> MHHHHHHHAVRASEISRVYEAYPEKKATLYFLVLGFLALIVGSLFGPFQALNYGNVDAYPLLKRLLPFVQSYYQGLTLHGVLNAIVFTQLFAQAIMVYLPARELNMRPNMGLMWLSWWMAFIGLVVFALPLLANEATVLYTFYPPLKGHWAFYLGASVFVLSTWVSIYIVLDLWRRWKAANPGKVTPLVTYMAVVFWLMWFLASLGLVLEAVLFLLPWSFGLVEGVDPLVARTLFWWTGHPINYFWLLPAYAIIYTILPKQAGGKLVSDPMARLAFLLFLLLSTPVGFHHQFADPGIDPTWKMIHSVLTLFVAVPSLMTAFTVAASLEFAGRLRGGRGLFGWIRAL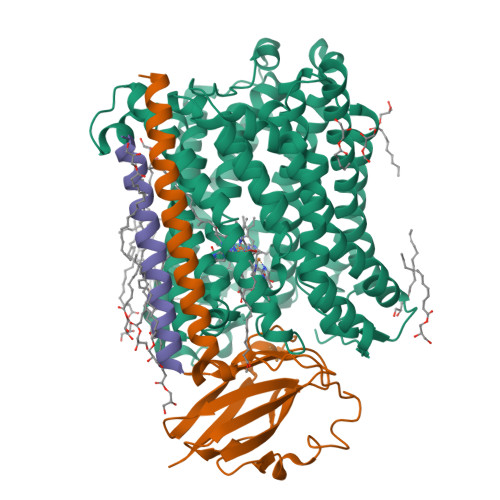PWDNPAFVAPVLGLLGFIPGGAGGIVNASFTLDYVVHNTAWVPGHFHLQVASLVTLTAMGSLYWLLPNLTGKPISDAQRRLGLAVVWLWFLGMMIMAVGLHWAGLLNVPRRAYIAQVPDAYPHAAVPMVFNVLAGIVLLVALLLFIYGLFSVLLSRERKPELAEAPLPFAEVISGPEDRRLVLAMDRIGFWFAVAAILVVLAYGPTLVQLFGHLNPVPGWRLW;> MVDEHKAHKAILAYEKGWLAFSLAMLFVFIALIAYTLATHTAGVIPAGKLERVDPTTVRQEGPWADPAQAVVQTGPNQYTVYVLAFAFGYQPNPIEVPQGAEIVFKITSPDVIHGFHVEGTNINVEVLPGEVSTVRYTFKRPGEYRIICNQYCGLGHQNMFGTIVVKE;> MEEKPKGALAVILVLTLTILVFWLGVYAVFFARG> SNATFLELVEVPCNSVHVQGVMTPNQMVKVTGAGWDNGVLEFYVTRPTKTGGDTSRSHLASIMCYSKDIDGVPSDKAGKCFLKRFSGEDSSEIDEKEVSLPIKSHNDAFMFVCSSNDGSALQCDVFALDNTNSNDGWKVNTVDLGVSVSPDLAFGLTADGVKVKKLYASSGLTAINDDPSLGCKA;> SNAGASCTYVWSDWNKCVCPMGYQARHAAVKFDYRNKPCDLPTFETKACSCGETNPVP

Microneme protein 2 (MIC2) and MIC2-associated protein (M2AP) play crucial roles in the gliding motility and host cell invasion of Toxoplasma gondii. Complex formation between MIC2 and M2AP is required for maturation and transport from the microneme to the parasite surface. MIC2 contains a von Willebrand factor type A (VWA) domain and six tandem thrombospondin type 1 repeat (TSR) domains in its ectodomain. In this study, we report crystal structures of M2AP alone and in complex with TSR6.

The TSR6–M2AP complex structure was solved using the M2AP crystal structure as a search template, and the TSR6 domain was manually built. Like other TSR domains, TSR6 in the complex has three parallel strands, with a stack of aromatic and basic residues forming π-cation bonds on the layered side, although the number of stacked residues in the layer is lesser in TSR6 than in typical TSR domains. Notably, a presumably layered residue, Tyr-602, adopts a conformation out of the layer, and a water molecule is positioned within the layer and hydrogen bonds to TSR6 residues Thr-601 and Pro-635. The complex structure reveals that the rod-like TSR6 domain binds through its non-layered side onto the hydrophobic face of the M2AP β-domain. The TSR6–M2AP interface buries a total of 1460 Å2 of accessible surface area. At the center of the binding interface, Lys-72 of M2AP forms a hydrogen bond interaction with both His-620 and the main-chains of Ala-621 and Thr-636. The His-620 of TSR6 additionally forms extensive hydrophobic interactions with M2AP residues Met-70, Met-153, Val-155, and Phe-169. At one edge of the interface, Trp-180 of M2AP inserts into a valley contributed by TSR6 ribbon residues Tyr-602 through Ser-605 and hydrogen bonds to the main-chain of Val-603. Remarkably, the H620A mutant decreased binding by >5000-fold, showing that His-620 is a hotspot in the binding interface. Furthermore, there is an attenuated peak at −61.50 ppm in the spectra of the complex, which can be assigned to a small population of layered state for either free TSR6 or in complex with M2AP, because the layered state of tfmF602 shares identical environment with or without M2AP. These NMR findings support the notion that Tyr-602 undergoes conformational equilibration between two states, and that binding to M2AP shifts the equilibrium towards the flipped-out state in which the Tyr-602 participates in the interface.> KSGKPSGEMDEVGVQKCKNALKLPVLEVLPGGGWDNLRNVDMGRVMELTYSNCRTTEDGQYIIPDEIFTIPQKQSNLEMNSEILESWANYQSSTSYSINTELSLFSKVNGKFSTEFQRMKTLQVKDQAITTRVQVRNLVYTVKINPTLELSSGFRKELLDISDRLENNQTRMATYLAELLVLNYGTHVTTSVDAGAALIQEDHLRASFLQDSQSSRSAVTASAGLAFQNTVNFKFEENYTSQNVLTKSYLSNRTNSRVQSIGGVPFYPGITLQAWQQGITNHLVAIDRSGLPLHFFINPNMLPDLPGPLVKKVSKTVETAVKRYYTFN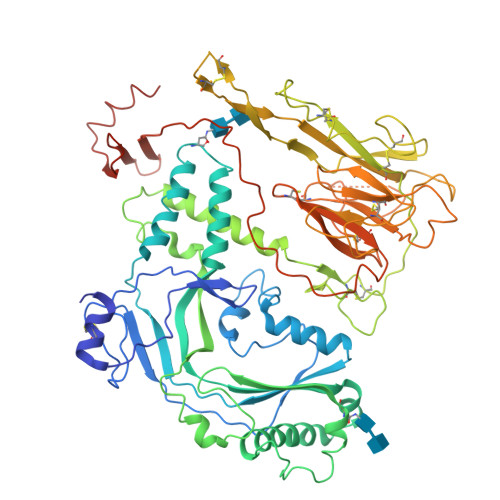TYPGCTDLNSPNFNFQANTDDGSCEGKMTNFSFGGVYQECTQLSGNRDVLLCQKLEQKNPLTGDFSCPSGYSPVHLLSQIHEEGYNHLECHRKCTLKVFCKTVCEDVFQVAKAEFRAFWCVASSQVPENSGLLFGGLFSSKSINPMTNAQSCPAGYFPLRLFENLKVCVSQDYELGSRFAVPFGGFFSCTVGNPLVDPAISRDLGAPSLKKCPGGFSQHPALISDGCQVSYCVKSGLFTGGSLPPARLPPFTRPPLMSQAATNTVIVTNSENARSWIKDSQTHQWRLGEPIELRRAMNVIHGDGGGLSHHHHHH> MKKLLTLACATMLTPVLAHGAFQLDSRYQDNDGDLIADIPSDESKLVDPSTLVFAYTPVEDPAVYKEVWSEFLDHLAETTGKNVQFFPVQSNAAQIEAMRAGRLHIAGFNTGSNPLAVACAGFRPFTMMAAADGSFGYEMEIISYPGSGVNDVEDIRGGELAFTSQTSNSGFKAPSAILKADYNMIAGEDFEPVFSGKHDNSILGVANRDYKAAAVANSVLNRMLSRDVVSEDQIVSLYKSQTFPTTGYGIAHNLTPELQEKIQDAFFSFNWEGTALEEEFSKSGEAQFVPITFKNHWEVIRKIDAANGVAYNCRHHHHH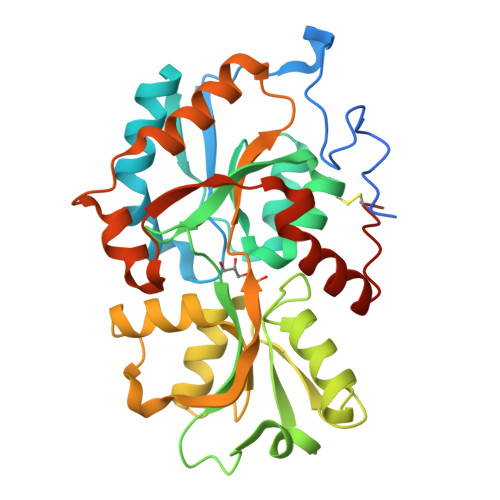H> NDPISNAIENAVSTLADTTISRVTAANTAASSHSLGTGRVPALQAAETGASSNASDENLIETRCVMNRNGVNEASVEHFYSRAGLVGVVEVKDSGTSQDGYTVWPIDVMGFVQQRRKLELSTYMRFDAEFTFVSNLNDSTTPGMLLQYMYVPPGAPKPDGRKSYQWQTATNPSIFAKLSDPPPQVSVPFMSPASAYQWFYDGYPTFGEHKQATNLQYGQCPNNMMGHFAIRTVSESTTGKNVHVRVYMRIKHVRAWVPRPFRSQAYMVKNYPTYSQTISNTAADRASITTTDYEGGVPANPQRTF;> MGAQVSAQKSGTHETGNIATEGSTI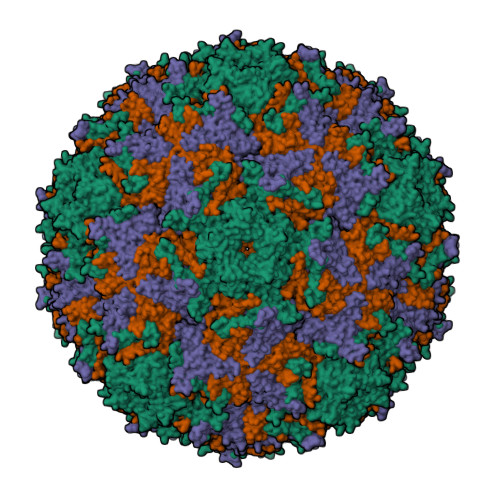NFTNINYYKDSYAASASRQDFTQDPTKFTSPVLDAIKEAAAPLQSPSVEACGYSDRVAQLTVGNSTITTQEAANIVLSYGEWPGYCPSTDATAVDKPTRPDVSVNRFYTLSTKSWKTESTGWYWKFPDVLNDTGVFGQNAQFHYLYRSGFCMHVQCNASKFHQGALLVVVIPEFVVAASSPATKPNGQGLYPDFAHTNPGKEGQVFRDPYVLDAGIPLSQALVFPHQWINLRTNNCATIIMPYVNALPFDSALNHSNFGLAVIPISPLKYCNGATTEVPITLTIAPLNSEFSGLRQAIKQ;> GLPTELKPGTNQFLTTDDGTSPPILPGFEPTPLIHIPGEFTSLLDLCRIETILEVNNTTGTTGVNRLLIPVRAQNNVDQLCASFQVDPGRNGPWQSTMVGQICRYYTQWSGSLKVTFMFTGSFMATGKMLIAYTPPGSAQPTTREAAMLGTHIVWDFGLQSSVTLVIPWISNTHFRAVKTGGVYDYYATGIVTIWYQTNFVVPPDTPSEANIIALGAAQENFTLKLCKDTDEIRQTAEYQ>[60x]SGVGHSTGNYNNRTEFYYHGDEVTIVCHSSRHIHLNMSESEEYKIYDTDRGPRFPTDQTLQGRDTINDSYHAQVETPWFLINPNSWGTWMNPADFQQLTTTCREVTLEHLDQTLDNIVIKTVSKQGSGAEETTQYNNDLTALLQVALDKSNQLPWVADNMYLDSLGYIPWRPCKLKQYSYHVNFWNTIDIISGPQQNQWQQVKKEIRWDDLQFTPIETTTEIDLLRTGDSWTSGPYKFNTKPTQLSYHWQSTRHTGSVHPTDPPNAIGQQGQNIRDINGWQWGDRSDPMSAATRVSNFHIGYSWPEWRIHYGSGGPAINPGAPFSQAPWSTDPQVRLTQGASEKAIFDYNHGDDDPAHRDQWWQNNLPIT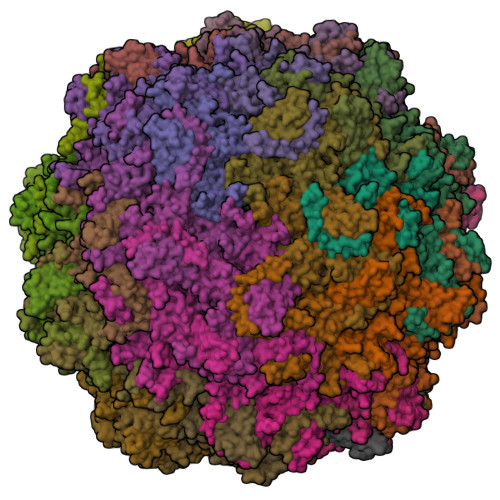GQTNWAPKNAHQANLSSNVPSRQEFWTQDYHNTFGPFTAVDDVGIQYPWGAIWTKTPDTTHKPMMSAHAPFICKDGPPGQLLVKLAPNYTENLQTDGLGNNRIVTYATFWWTGKLILKGKLRLPRQFNLYNLPGRPRGTEAKKFLPNEIGHFELPFMPGRCMPNYTM> MIVLFVDFDYFYAQVEEVLNPSLKGKPVVVCVFSGRFEDSGAVATANYEARKFGVKAGIPIVEAKKILPNAVYLPMRKEVYQQVSSRIMNLLREYSEKIEIASIDEAYLDISDKVRDYREAYNLGLEIKNKILEKEKITVTVGISKNKVFAKIAADMAKPNGIKVIDDEEVKR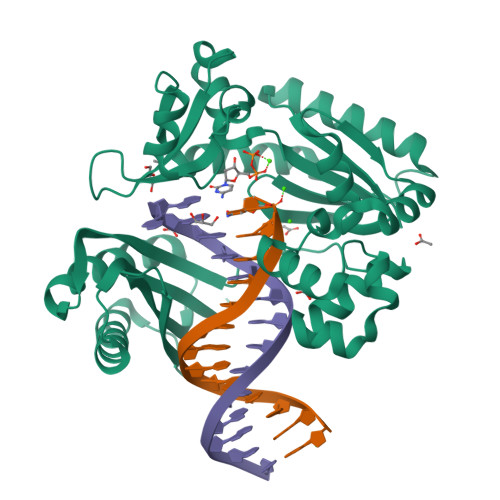LIRELDIADVPGIGNITAEKLKKLGINKLVDTLSIEFDKLKGMIGEAKAKYLISLARDEYNEAIRTRVRKSIGRIVTMKRNSRNLEEIKPYLFRAIEESYYKLDKRIPKAIHVVAVTEDLDIVSRGRTFPHGISKETAYSESVKLLQKILEEDERKIRRIGVRFSKFIEA> MGWSDHDELSTDTTLHEEKFRIEPVPVHHQLDILKIAVSENYKTFASVGLDRCLVVWDLRQWCTKLVLSKEQMPRTLKAIALDPQGNYVSLFSKDTLFILNVESPSLMLQHSYHCKPNSKLNVFWMPGTHKDDEWKNFELVVVESSGEIQVFSLTIEIEGADIALVEKFQLSSPIIKSISIVSPTANRIACLTESGEVTVYSKKGPVWSPKILSQNKNYLTETKKDIYGIAMADIL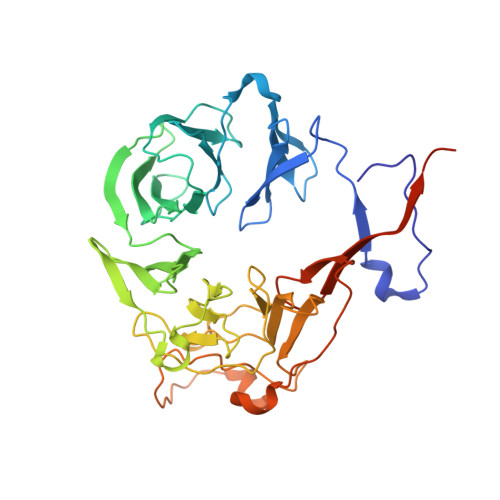FLARDSGVDMIDLKNDELLHSFTLPPIKVNTFSVGVSNSRFVNGQFRVSSISFCFTHAVTEKVLYYYYGNESNESYIILNKWDQQPNLVDVHDPDNSLASLTFDELQENIHEVEDASESVMSSDGLYIFGMRRKSSSGISPTADEKNEDNGFTLRNRKLR Delafloxacin is a potent anionic fluoroquinolone approved for the treatment of respiratory infections that acts by trapping the DNA cleavage complexes of bacterial topoisomerase IV and gyrase. Topo IV is a tetrameric complex made up of two ParE and two ParC subunits that mediates unlinking of interlocked daughter chromosomes. Fluoroquinolones stabilise this complex which cellular processes convert into a lethal lesion, likely a frank double-stranded DNA break.

Co-crystallisation trials were set up to include the ParE30-ParC55 fusion protein, the strongly cleaved 18-mer E-site DNA duplex (present on the pneumococcal chromosome) or the 18-mer V-site DNA sequence (present in ColE1 plasmids) plus 2 mM delafloxacin to saturate drug binding. Crystals of the cleavage complex were obtained with both DNA duplexes and the structures were solved at 2.4 Å resolution by molecular replacement. The delafloxacin complex presents as a dimer with the two ParC55 breakage-reunion domains in a ‘closed’ conformation flanked by the two ParE30 metal binding TOPRIM domains, with a single DNA helix bound across the dimer interface. The ParE domains- formed of four parallel β-sheets and surrounding α-helices- plus the ParC winged helix domain (WHD) and ‘tower’ domains together form the protein groove that accommodates a single V-site (or E site DNA) duplex as the G-gate DNA. Protein binding induces a U-shaped bend in the DNA involving the symmetric minor groove intercalation of the two ParC I170 sidechains. A magnesium-chelated delafloxacin molecule is intercalated into the wedge-shaped space between the -1 and +1 nucleotides at each end of the 4-bp staggered DNA break site introduced into the 18-mer V-site duplex by nucleophilic attack of the two ParC Y118 residues. The 5′-phosphates at the ends of the DNA break are covalently linked to ParC Y118 residues confirming capture of the cleavage complex. Analysis of DNA conformation using the w3DNA programme revealed that all regions of the drug-captured G-gate DNA adopt a B-form helix.

>[2x]MKNKKDKGLLSGKLTPAQSKNPAKNELYLVEGDSAGGSAKQGRDRKFQAILPLRGKVINTAKAKMADILKNEEINTMIYTIGAGVGADFSIEDANYDKIIIMTDADTDGAHIQTLLLTFFYRYMRPLVEAGHVYIALPPLYKMSKGKGKKEEVAYAWTDGELEELRKQFGKGATLQRYKGLGEMNADQLWETTMNPETRTLIRVTIEDLARAERRVNVLMGDKVEPRRKWIEDNVKFTLEEATVFHMSNIQNMSLEDIMGERFGRYSKYIIQDRALPDIRDGLKPVQRRILYSMNKDSNTFDKSYRKSAKSVGNIMGNFHPHGDSSIYDAMVRMSQNWKNREILVEMHGNNGSMDGDPPAAMRYTEARLSEIAGYLLQDIEKKTVPFAWNFDDTEKEPTVLPAAFPNLLVNGSTGISAGYATDIPPHNLAEVIDAAVYMIDHPTAKIDKLMEFLPGPDFPTGAIIQGRDEIKKAYETGKGRVVVRSKTEIEKLKGGKEQIVITEIPYEINKANLVKKIDDVRVNNKVAGIAEVRDESDRDGLRIAIELKKDANTELVLNYLFKYTDLQINYNFNMVAIDNFTPRQVGIVPILSSYIAHRREVILARSRFDKEKAEKRLHIVEGLIRVISILDEVIALIRASENKADAKENLKVSYDFTEEQAEAIVTLQLYRLTNTDVVVLQEEEAELREKIAMLAAIIGDERTMYNLMKKELREVKKKFATPRLSSLEDTAKALEHHHHHH> LICVN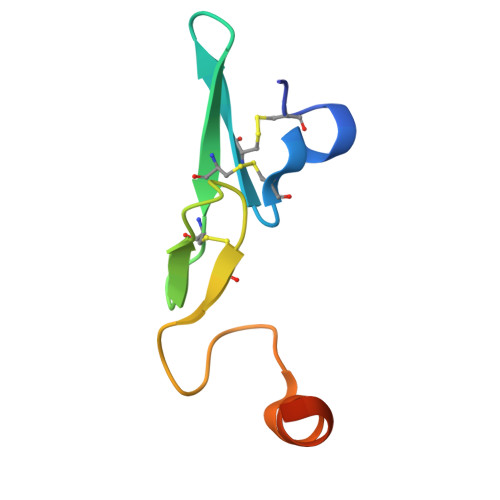ENGGCEQYCSDHTGTKRSCRCHEGYSLLADGVSCTPTVEYPCGKIPILEKRNASKPQGR Macrolide resistance is abundant in pathogenic bacteria, and is most often the result of GTP-dependent macrolide kinases (Mph), ribosomal methyltransferases, or efflux pumps. Mph enzymes inactivate macrolides by phosphorylating the 2′-OH of the essential dimethylamino sugar, preventing it from binding the ribosome, and providing the chemical rationale for the resistance phenotype. Mph enzymes are therefore adaptable resistance enzymes with complex evolutionary paths.

While the MphA, MphB, and MphH structures are very similar, we observed structural distinctions in all three enzymes that localized to the (a) NPL, (b) β-hairpin insert, and (c) multiple residues in the macrolide-binding cleft. As we observed in MphH, the NPL, and β-hairpin regions of both MphA and MphB adopt different conformations with macrolide binding. Consistent with the flexibility of MphH in our crystal structure, these observations highlight that conformational changes in these key regions of Mph enzymes play a role in macrolide substrate binding.

>[2x]MPEDLDALLDLAARHGLDLDGGTLRTEEIGLDFRVAFARAHDGGDWVLRLPRRPDVLERAAVEGRLLAMLAPHLDVAVPDWRISTSELIAYPLLPGSPGLTVAADGEVSWHVDMASTVYARSLGSVVAQLHAVDAEAAAATGIEVRSPAQVRGAWRQDLARVGAEFEIAPALRERWEAWLADDGCWPGHSVLTHGELYPAHTLVEDERITAVLDWTTAAVGDPAKDLMFHQVSAPSAIFEVALQAYAEGGGRPWPGLARHCTEMFSAAPLGYGLYALATGEAAHREAAAAALNPPEER>AEKGVYAHYMLKEIHEQPAVMRRIIQEYQDAEGNLKIDQDIINDVKEADRIYVIAAGTSYHAGLVGKEFLEKWAGVPTEVHVASEFVYNMPLLSEKPLFVYISQSGETADSRAVLVETNKLGHKSLTITNVAGSTLSREADHTLLLHAGPEIAVASTKAYTAQIAVLSILSQIVAKEHGREADIDLLRELAKVTTAIEAIVDDAPIMEQIATDFLETTRNAFFIGRTIDYNVSLEGALKLKEISYIQAEGFAGGELKHGTIALIEDGTPVVALATQENVNLSIRGNVKEVVARGAHPCIISMEGLEKEGDTYVIPHVHELLTPLVSVVAL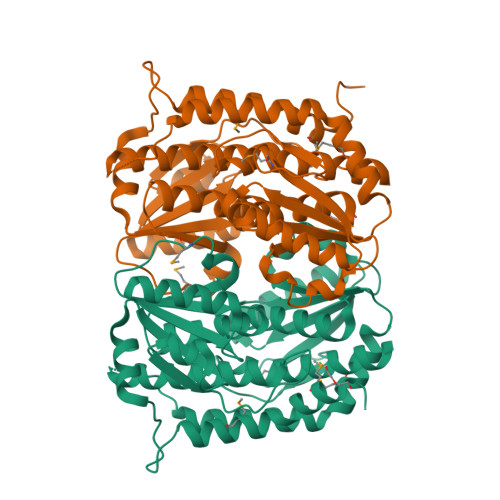QLISYYAALHRDLDVDKPRNLAKSVTVE[2x]> MFGVTRKLLGELSEYVEVNEKGMPKPQALSLWNMPYAKRRALTKFARGVRWQFI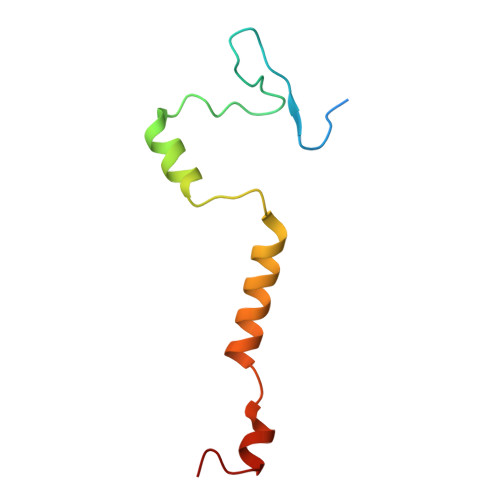VLFIALYNFKNRDDSHLLRRGAYN>GSVIRHFLRDDDLSPAEQAEVLELAAELKKDPVSRRPLQGPRGVAVIFDKNSTRTRFSFELGIAQLGGHAVVVDSGSTQLGRDETLQDTAKVLSRYVDAIVWRTFGQERLDAMASVATVPVINALSDEFHPCQVLADLQTIAERKGALRGLRLSYFGDGANNMAHSLLLGGVTAGIHVTVAAPEGFLPDPSVRAAAERRAQDTGASVTVTADAHAAAAGADVLVTDTWTSMGQENDGLDRVKPFRPFQLNSRLLALADSDAIVLHCLPAHR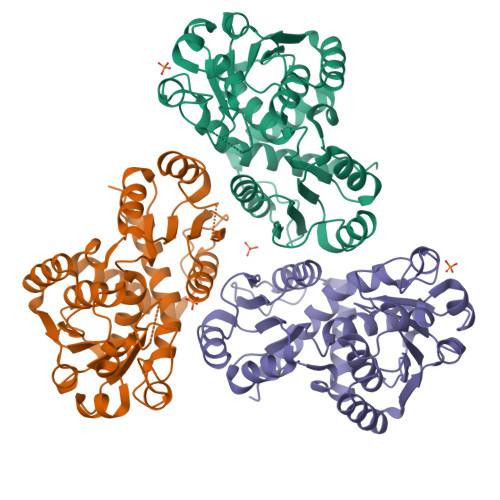GDEITDAVMDGPASAVWDEAENRLHAQKALLVWLLERS[6x]Here, a series of new methods are presented based on the use of a low X-ray-background film as a crystallization support and a photoablation laser that enable the automation of major operations required for the preparation of crystals for X-ray diffraction experiments. In this approach, the controlled removal of the mother liquor before crystal mounting simplifies the cryocooling process, in many cases eliminating the use of cryoprotectant agents, while crystal-soaking experiments are performed through diffusion, precluding the need for repeated sample-recovery and transfer operations. We have previously shown that the transfer of crystals to X-ray data-collection pins can be automated through the so-called CrystalDirect approach, which relies on the use of a thin, low X-ray-background film as a crystallization support from which crystals are recovered by excising the film with a laser beam and attaching it to an X-ray data-collection pin. The CrystalDirect system enables the automation of sample mounting and cryocooling and can contribute to closing the automation gap that currently exists between crystallization and X-ray data collection.

As an initial validation, crystals of proteinase K, thaumatin and lysozyme were prepared in CrystalDirect plates. These crystals grow from solutions that typically require the addition of cryoprotectants when mounted manually. The CrystalDirect approach provides a robust method for automated sample cryocooling without the need to screen for cryoprotectant agents, which is often a critical step in protein crystallography.

> AAQTNAPWGLARISSTSPGTSTYYYDESAGQGSCVYVIDTGIEASHPEFEGRAQMVKTYYYSSRDGNGHGTHCAGTVGSRTYGVAKKTQLFGVKVLDDNGSGQYSTIIAGMDFVASDKNNRNCPKGVVASLSLGGGYSSSVNSAAARLQSSGVMVAVAAGNNNADARNYSPASEPSVCTVGASDRYDRRSSFSNYGSVLDIFGPGTSILSTWIGGSTRSISGTSMATPHVAGLAAYLMTLGKTTAASACRYIADTANKGDLSNIPFGTVNLLAYNNYQA(E)-3-(1H-indol-3-yl)-2-oxidanyl-but-2-enoic acid | 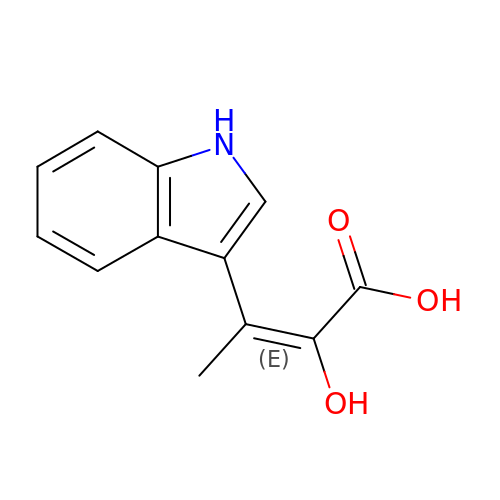C12 H11 N O3 | PPGRYTGRWGDNAP-YRNVUSSQSA-N> 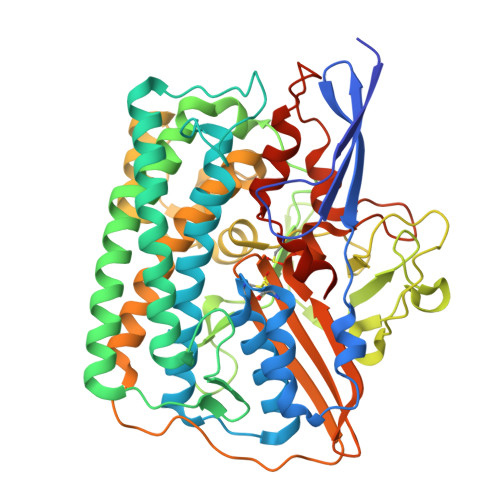WSHPQFEKGATGRTTIAIDPVTRIEGHLKAEVVVENGKVVDARLSGGMYRGFETILRGRDPRDASQIVQRICGVCPTAHSTASVLALDEAFGAKVPNNGRITRNLIFGANYLQSHILHFYHLSAQDFVQGPDTAPFVPRFPKSDLRLSKELNKAGVDQYIEALEVRRICHEMVALFGGRMPHVQGQVVGGATEIPTKEKLVEYAARFKKVRDFVEQKYVPVVYTIGSKYKDMFKVGQGFKAALCVGAFPLDNSGKKHLFMPGVYAKGKDMPFDPSKIKEYVKYSWFAEETTGLNYKEGKTIPAPDKAGAYSFVKAPRYDGLSLEVGPLARMWVNNPELSPVGKKLLKDLFGISAKKFRDLGEEAAFSLMGRHVARAEETYYMLGAIEGWLKEIKAGEDTVVMPAVPASAEGTGFTEAPRGSLLHYVKVKDSKIDNYQIVSASLWNCNPRDDMGQRGAVEEALIGIPVDDIQNPVNVARLIRAFDPCLGCAVHVLHAESGKVAVIEVK>[4x]MPHHIVIVEDEPVTQARLQSYFTQEGYTVSVTASGAGLREIMQNQSV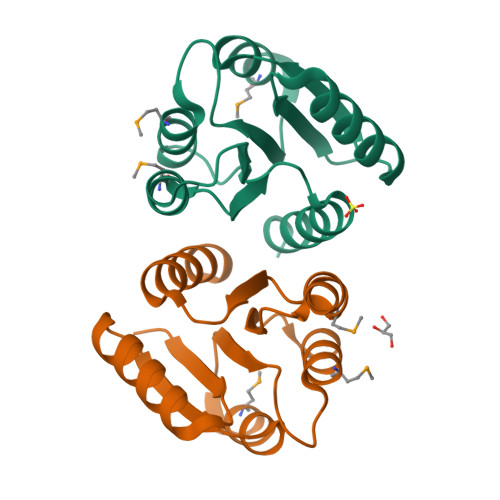DLILLDINLPDENGLMLTRALRERSTVGIILVTGRSDRIDRIVGLEMGADDYVTKPLELRELVVRVKNLLWRIDQ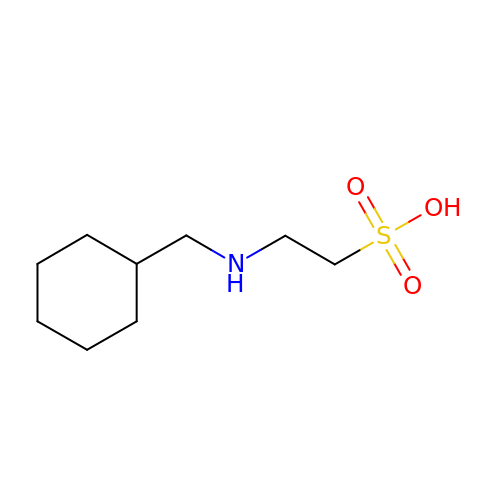2-[(cyclohexylmethyl)amino]ethanesulfonic acid | C9 H19 N O3 S | UMTSMLKBBCGVNJ-UHFFFAOYSA-N{3-[(4-amino-2-methylpyrimidin-5-yl)methyl]phenyl}methanol | C13 H15 N3 O | 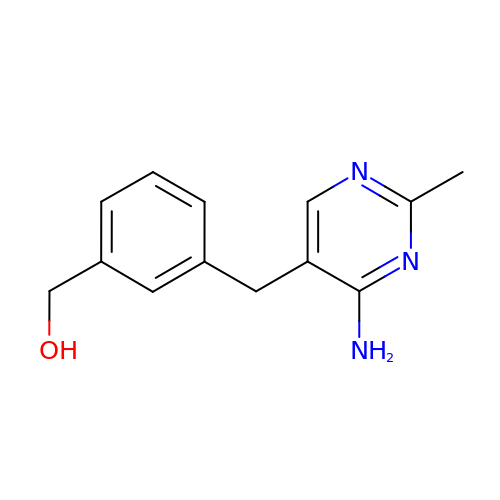WCYNVVXZGIHJNV-UHFFFAOYSA-N> MNRQVIEFSKYNPSGNMTILVHSKHDASEYASIANQLMAATHVCCEQVGFIESTQNDDGNDFHLVMSGNEFCGNATMSYIHHLQESHLLKDQQFKVKVSGCSDLVQCAIHDCQYYEVQMPQAHRVVPTTINMGNHSWK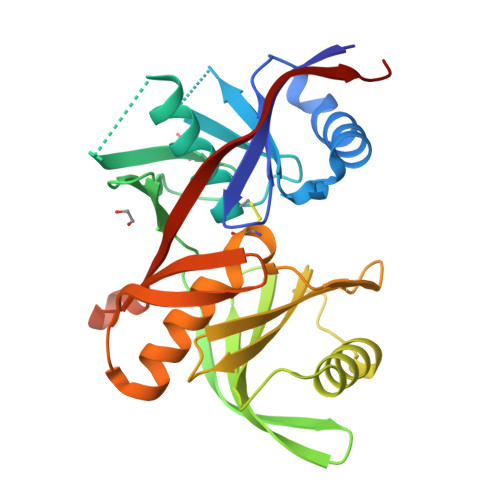ALEIIYETYVHYVIPVKQVTTEIQHLVEAFVREQQWSHKYKTVGMMLFDEQRQFLQPLIYIPEIQSLIWENSCGSGTASIGVFNNYQRNDACKDFTVHQPGGSILVTSKRCHQLGYQTSIKGQVTTVATGKAYIELEHHHHHH>GSHMATFLIKHKASGKFLHPKGGSSNPANDTNLVLHSDIHERMYFQFDVVDERWGYIKHAASGKIVHPLGGKADPPNETKLVLHQDRHDRALFAMDFFNDNIIHKAGKYVHPKGGSTNPPNETLTVMHGDKHGAMEFIFVSPKNKDKRVLVYV[2x]

MytiLec, a lectin isolated from the Mediterranean mussel Mytilus galloprovincialis, was identified through a study of marine organisms and their adaptation to different habitats and environmental systems, and shown to bind α-D-galactose and N-acetyl-α-D-galactosamine (α-GalNAc). The structure is well ordered, with the entire main-chain of each monomer visible in the 2mFo-DFc electron density map, revealing a β-trefoil fold consisting of three related sub-domains. MytiLec is somewhat unusual in binding ligand at each subdomain, and it forms a dimer in solution, giving a total of six ligand sites per protein.

Apo-MytiLec crystallised in space-group P21, and diffracted to 1.1 Å resolution. The lack of an obvious search model led us to determine phases using a heavy atom derivative, which was aided by the strong diffraction of the physically robust crystals. Two monomers of MytiLec are found in the asymmetric unit, and the model shows expected geometrical features and has no Ramachandran outliers. Several N-terminal residues remaining from the thrombin-cleavable tag are also present in the apo-MytiLec electron density map, so that chain numbering of the apo structure starts at -1 or -3. Least-squares fitting the Cα atoms of residues 1 to 149 of each chain in the apo-MytiLec model gives a rmsd of 0.27 Å. Overlaying 37 central Cα atoms of individual sub-domains from within the same chain gives rmsd values no higher than 0.6 Å, indicating a high degree of internal symmetry. The two monomers in the asymmetric unit are closely associated by hydrophobic interactions and hydrogen bonds, as shown in Supplementary Tables S1 and S2. PISA18 reports the buried interface area between MytiLec monomers to be about 740 Å2 per chain. Two adjacent phenylalanine residues, Phe 93 and Phe 94, sit opposite their symmetry mates at the dimer interface. MytiLec was originally reported to be a monomer in solution on the basis of gel filtration but analytical ultracentrifugation confirms the protein is a tightly-bound dimer, and mutation of Phe 93 and Phe 94 blocks dimerisation. In order to observe any changes in the protein on ligand binding, both the apo and GalNAc complex structures were determined. Both the apo crystal and the co-crystal with ligand were cryo-protected immediately prior to flash-cooling by soaking in mother liquor containing 25% glycerol.7-hydroxy-6-methylfuro[3,4-c]pyridin-1(3H)-one 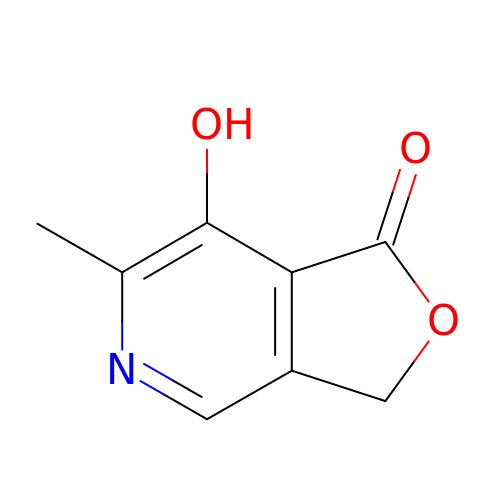| C8 H7 N O3 | HHPDVQLBYQFYFA-UHFFFAOYSA-N>[4x]MRGSHHHHHHGMASMRILLSNDDGVHAPGIQTLAKALREFADVQVVAPDRNRSGASNSLTLESSLRTFTFDNGDIAVQMGTPTDCVYLGVNALMRPRPDIVVSGINAGPNLGDDVIYSGTVAAAMAGRHLGFPALAVSLNGYQHYDTAAAVTCALLRGLSREPLRTGRILNVNVPDLPLAQVKGIRVTRCGSRHPADK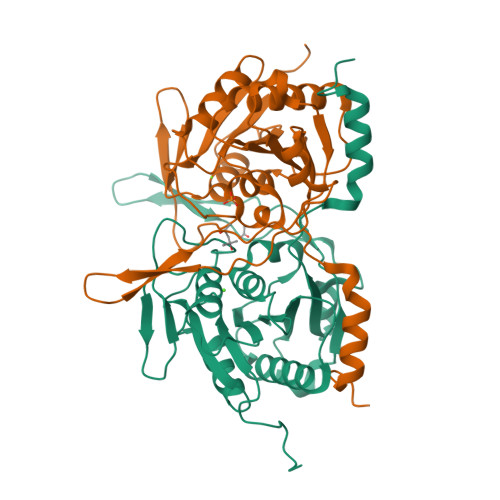VIPQEDPRGNTLYWIGPPGDKYDAGPDTDFAAVDEGYVSVTPLHVDLTAASAHDVVSDWLDSVGVGTQW>MMQFTMSGTMLRFDETTLRFSFSRDGATWSGCDGIEPQLTREDRSFSFAGAATVTHERIETGTGVGVRSVFAGFAGADYAFETYIWIERSSGDVLCEWVPLRECGAEPRIDRVLWPAPLSFDRADAHDVTLITHEQGVMIPNSWPTEVGTDAVSFGGRFETAGGYMPWFAQLRSDGHAYIAICETPWNAGYDIDHPAGGPYTHVGMWFEPSLGRMDYRRVVRYRLLDHADHTAICKTYRAYVNERGRLRTLAEKAARNPSVRDLLGRSWVHVGIKTNVQPDSSFYDPAQPGKNDSLVTFAQRERQMRTLHEMGAGRLYLHLDGWAQPGYDNGHPDYLPACREAGGWKGMKSLIDACHEQGDLFGTHDQYRDYYFAARTFDPRNAIRLADGTMPEHAMWAGGRQTYLCAELAPDYVRRNFSEIATHGIVLDCAYLDVFTCNEGDECSHPEHRMTRRECYERRAECFEYLLAHGILTSSEEVSDWAVPSLVFCHYAPYDFQMRSPDAPRHGIPVPLYNLVYHDCVIQPWMMDRVAGGDDYMLYALLNGGAPYLIRD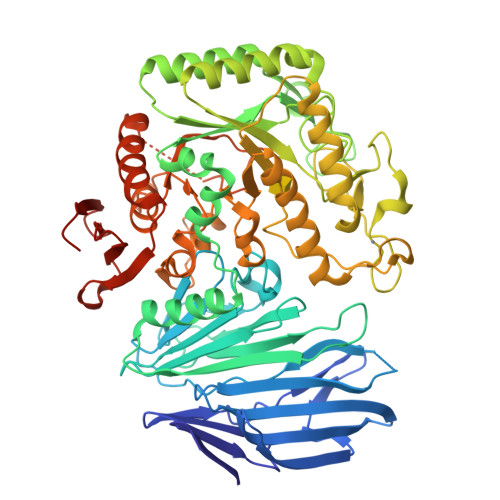AAYAGMDGDMNAALRARTENDIERCAVVAGLHRRVGMQELVRHDLVGGDPLVQRSVFADGTAVTCDFHAQTYEVAANGSHHHHHHH[2x]>[2x]MGSSHHHHHHSSGETVRFQGHMNLSQLSFHRVDQKEITQLSHLGQGTRTNVYEGRLRSEGSGDPEEGKMDDEDPLVPGRDRGQELRVVLKVLDPSHHDIALAFYETASLMSQVSHTHLAFVHGVCVRGPENIMVTEYVEHGPLDVWLRRE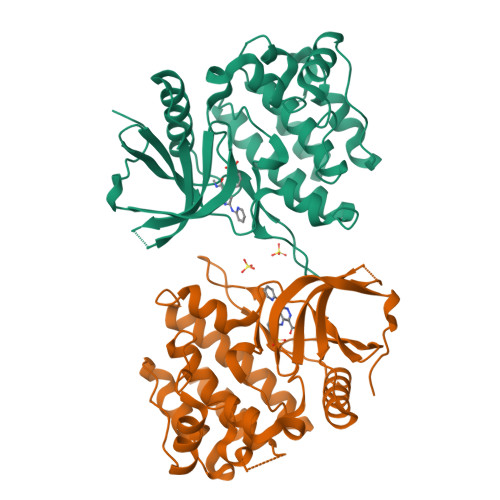RGHVPMAWKMVVAQQLASALSYLENKNLVHGNVCGRNILLARLGLAEGTSPFIKLSDPGVGLGALSREERVERIPWLAPECLPGGANSLSTAMDKWGFGATLLEICFDGEAPLQSRSPSEKEHFYQRQHRLPEPSCPQLATLTSQCLTYEPTQRPSFRTILRDLTRL N-({(1R,2R,3S)-2-(methylcarbamoyl)-3-[4-(phosphonooxy)phenyl]cyclopropyl}carbonyl)-L-valyl-L-aspartamide | C21 H30 N5 O9 P 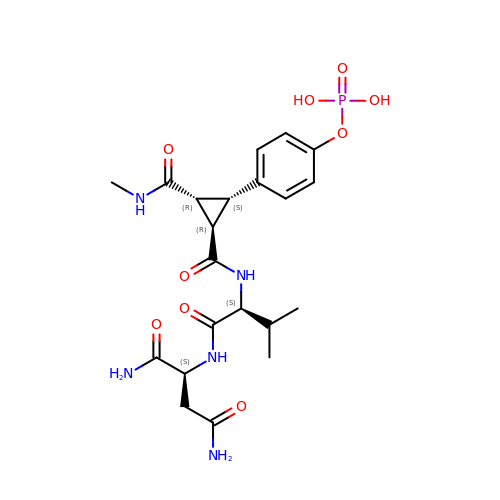| LVYNAUCEOQBVSW-RDDKANTKSA-N>[3x]ATPHINAEMGDFADVVLMPGDPLRAKYIAETFLED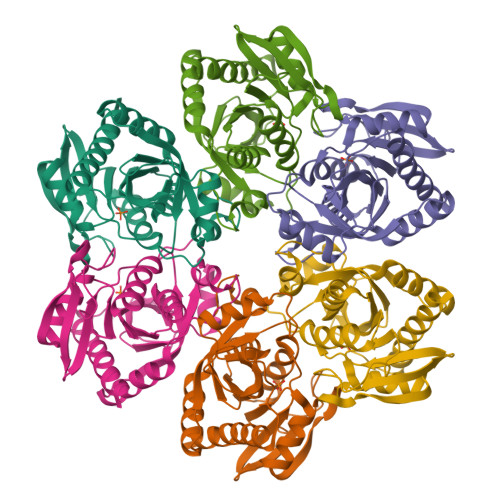AREVNNVRGMLGFTGTYKGRKISVMGHGVGIPSCSIYTKELITDFGVKKIIRVGSCGAVLPHVKLRDVVIGMGACTDSKVNRIRFKDHDFAAIADFDMVRNAVDAAKALGIDARVGNLFSADLFYSPDGEMFDVMEKYGILGVEMEAAGIYGVAAEFGAKALTICTVSDHIRTHEQTTAAERQTTFNDMIKIALESVLLGDKE> TENILRKSDEEIQKEITARVKALESMLIEQGILTTSMIDRMAEIYENEVGPHLGAKVVVKAW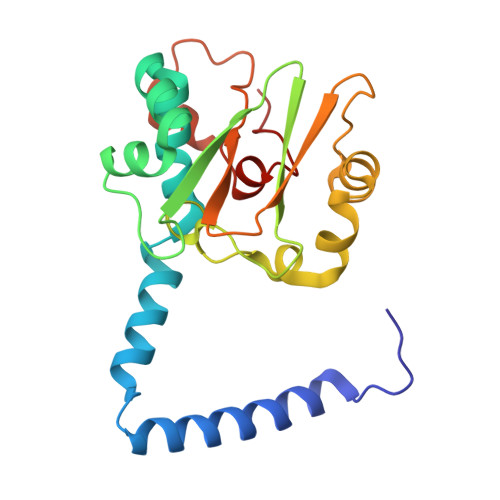TDPEFKKRLLADGTEACKELGIGGLQGEDMMWVENTDEVHHVVVCTLCSCTPWPVLGLPPNWFKEPQYRSRVVREPRQLLKEEFGFEVPPSKEIKVWDSSSEMRFVVLPQRPAGTDGWSEEELATLVTRESMIGVEPAKAV>[2x]MSEENVVYIGNKPVMNYVLAVVTQMNGGTSEVILKARGIAISRAVDVAEIVRNRFIPDIQIENIDICTEEIIGNEGTATNVSAIEIQLRKD

The Sac10b protein family, also named Alba, is generally regarded as a family of DNA-binding proteins that are highly conserved and widely distributed within the archaea. However, unlike typical Sac10b family proteins, Mth10b is an acidic protein which contains 13 acidic amino acid residues and only 8 basic residues, and its potential isoelectric point is only 4.56. However, electrophoretic mobility shift analysis (EMSA) showed that Mth10b does not bind to either DNA or RNA. Although Mth10b has no ability to interact with nucleic acids in vitro, the overall structure of Mth10b still closely resembles other Sac10b family DNA-binding proteins.

We have determined the crystal structure of M. thermoautotrophicum ΔH Mth10b at a resolution of 2.2 Å. The crystal structure of the Mth10b monomer is of mixed α/β type, and consists of two α-helices and four β-strands with a topology of β1-α1-β2-α2-β3-β4. The strands β1, β2 and β4 are parallel, while strand β3 is antiparallel to the other strands. This structure model covers 86 of the total 91 residues, and no electron density was observed for the four N-terminal residues or for C-terminal Asp91. Two adjacent asymmetric Mth10b monomers interact with each other side-by-side along the long dimension of the monomer, forming a dimer with a crystallographic two-fold axis perpendicular to the long dimension of the dimer. The overall structure of the Mth10b dimer resembles a body with two long, extending, flexible β-hairpin arms, agreeing well with the dimeric structures reported for typical members of the Sac10b family. Helix α2, and strands β3 and β4 are involved in dimerization, through hydrophobic interactions as well as hydrogen bonding. In addition, each monomer in the Mth10b structure contains four salt bridges: Glu31-Arg89, Lys35-Glu85, Arg37-Glu69, and Glu49-Arg52. Though Mth10b is an acidic protein, the concave surface of the molecule corresponding to the DNA-binding surface in Sso10b is dominated by positively-charged residues, but its positive electrostatic potential is much lower than that of Sso10b. The other three pairs of conserved positively-charged residues, namely Lys16, Arg44 and Arg83 in each Sso10b monomer, are substituted, respectively, in Mth10b by neutral residues Asn11, Ile39 and Thr77, suggesting that these three pairs of residues should be key to the interaction between typical Sac10b family proteins and DNA. Mth10b mutants N11K, I39R and T77R with the neutral residues changed to corresponding positively-charged residues acquired DNA-binding activity and the triple mutant N11KI39RT77R exhibited even higher DNA-binding activity.PRPP is formed from ATP and D-ribose-5-phosphate (R5P) by the phosphoribosyl pyrophosphate synthetases (PRSs). The human PRS family, which has 3 isoforms (hPRS1, hPRS2 and hPRS3), belongs to the class I PRSs that requires divalent metal ions such as Mg2+ as the activator, inorganic phosphate ion for activity, and ATP or dATP as the diphosphoryl donor. Due to the important role of PRPP in the nucleotide metabolic process, the stability of PRPP content is essential for cell physiology and is predominantly controlled by hPRS1, the ubiquitously expressed human PRPP synthetase. Mutations in hPRS1 affect vital cell functions and are related to many diseases and disorders.

We determined the crystal structures of the E43T, D65N, A87T, M115T and Q133P mutations at a resolution of 3.0 Å, 2.14 Å, 3.3 Å, 2.11 Å and 2.74 Å, respectively, with 2 molecules in each asymmetric unit. Overall, the structures of all the five structures are highly similar to that of the wild type PRS1 with RMSD listed in S2 Table. In the Q133P structure, the Gln133 replaced by Pro133 destroys the hydrogen bond interaction between Gln133 and Asp98 in the PRS1, which might reduce the restraint of the catalytic flexible loop. The MD simulation result indicates that there are fewer contacts between the Pro133 in Q133P mutant and the catalytic flexible loop. The Q133P mutant influences the catalytic flexible loop due to the loss of hydrogen bonds, consequently results in a loss of function.

>[2x]MPNIKIFSGSSHQDLSQKIADRLGLELGKVVTKKFSNQETCVEIGESVRGEDVYIVQSGCGEINDNLMELLIMINACKIASASRVTAVIPCFPYARQDKKDKSRAPISAKLVANMLSVAGADHIITMDLHASPIQGFFDIPVDNLYAEPAVLKWIRENISEWRNCTIVSPDAGGAKRVTSIADRLNVDFALIHKERKKANEVDRMVLVGDVKDRVAILVDDMADTCGTICHAADKLLSAGATRVYAILTHGIFSGPAISRINNACFEAVVVTNTIPQEDKMKHCSKIQVIDISMILAEAIRRTHNGESVSYLFSHVPLLEHHHHHH> SRPLSDQEKRKQISV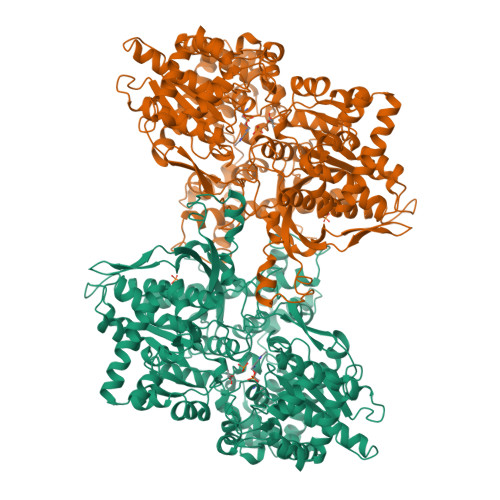RGLAGVENVTELKKNFNRHLHFTLVKDRNVATPRDYYFALAHTVRDHLVGRWIRTQQHYYEKDPKRIYYLSLEFYMGRTLQNTMVNLALENACDEATYQLGLDMEELEEIEEDAGLGNGGLGRLAACFLDSMATLGLAAYGYGIRYEFGIFNQKICGGWQMEEADDWLRYGNPWEKARPEFTLPVHFYGRVEHTSQGAKWVDTQVVLAMPYDTPVPGYRNNVVNTMRLWSAKAPNDFNLKDFNVGGYIQAVLDRNLAENISRVLYPNDNFFEGKELRLKQEYFVVAATLQDIIRRFKSSKFGCRDPVRTNFDAFPDKVAIQLNDTHPSLAIPELMRVLVDLERLDWDKAWEVTVKTCAYTNHTVIPEALERWPVHLLETLLPRHLQIIYEINQRFLNRVAAAFPGDVDRLRRMSLVEEGAVKRINMAHLCIAGSHAVNGVARIHSEILKKTIFKDFYELEPHKFQNKTNGITPRRWLVLCNPGLAEIIAERIGEEYISDLDQLRKLLSYVDDEAFIRDVAKVKQENKLKFAAYLEREYKVHINPNSLFDVQVKRIHEYKRQLLNCLHVITLYNRIKKEPNKFVVPRTVMIGGKPAPGYHMAKMIIKLITAIGDVVNHDPVVGDRLRVIFLENYRVSLAEKVIPAADLSEQISTAGTEASGTGNMKFMLNGALTIGTMDGANVEMAEEAGEENFFIFGMRVEDVDRLDQRGYNAQEYYDRIPELRQIIEQLSSGFFSPKQPDLFKDIVNMLMHHDRFKVFADYEEYVKCQERVSALYKNPREWTRMVIRNIATSGKFSSDRTIAQYAREIWGVEPSRQRLPAPDEKIP> YPFVEPI;> VVGGTEAQRNSWPSQISLQYRSGSSWAHTCGGTLIRQNWVMTAAHCVDRELTFRVVVGEHNLNQNNGTEQYVGVQKIVVHPYWNTDDVAAGYDIALLRLAQSVTLNSYVQLGVLPRAGTILANNSPCYITGWGLTRTNGQLAQTLQQAYLPTV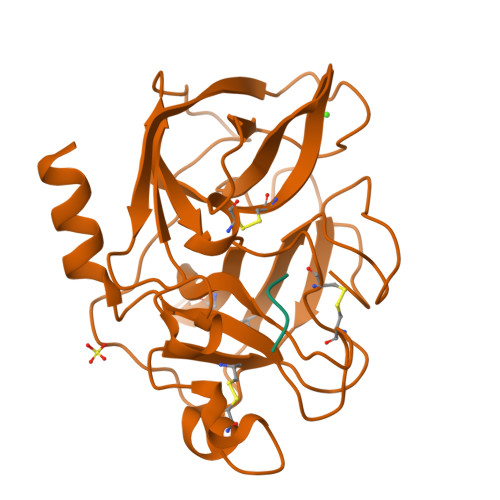DYAICSSSSYWGSTVKNSMVCAGGDGVRSGCQGDSGGPLHCLVNGQYAVHGVTSFVSRLGCNVTRKPTVFTRVSAYISWINNVIASN>[2x]GPLGRGREEKAPEEPQPVKMPENNSVVEATWNDVQLEDSLGMEVGYRLIPMVDFQQDGELLGRIRSIRKKFAQDMGFLPPVVHIRDNMDLQPARYRILMKGVEIGSGDAYP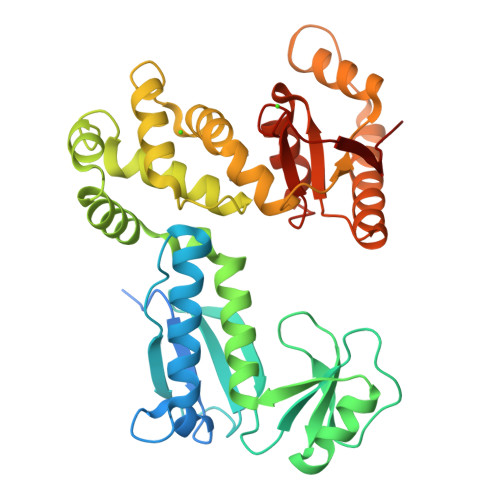GRWLAINPGTAAGTLPGEKTVDPAFGLDAIWIESALKEQAQIQGFTVVEASTVVATHLNHLIGQFSAELFGRQEAQQLLDRVSQEMPKLTEDLVPGVVTLTTLHKVLQNLLAEKVPIRDMRTILETLAEHAPLQSDPHELTAVVRVALGRAITQQWFPGNEEVQVIGLDTALERLLLQALQGGGGLEPGLADRLLAQTQEALSRQEMLGAPPVLLVNHALRPLLSRFLRRSLPQLVVLSNLELSDNRHIRMTATIGGK>GPTEEQAAENWRDAMKTELQTIRTEIQEETARRQEELNAQNLVKMQELMSNFFQKITI[8x]

C. elegans SAS-6 physically interacts with SAS-5, a protein that shuttles rapidly between the cytoplasm and centrioles throughout the cell cycle. The presence of SAS-6 and SAS-5 at centrioles is essential for formation of the central tube, a cylindrical structure at the core of the emerging centriole. Overall, these findings led us to conclude that the segment between residues 125–265 contains two independently folded domains and encompasses all structured elements of SAS-5.

Native crystals of SAS-5CC diffracted to 1.8 Å resolution, whilst phases for structure solution were determined by single anomalous dispersion (SAD) using trimethyl lead acetate derivatized crystals. The structure of SAS-5CC suggested a parallel trimeric coiled coil, although this arrangement is distorted by crystal packing that intercalates the ends of successive triple helical bundles. To correct for these distortions, we performed molecular dynamics (MD) simulations starting from the crystallographic structure of SAS-5CC, which rapidly converged to a trimeric coiled-coil structure. SEC-MALS analysis of a slightly longer coiled-coil construct (SAS-5CC-L, residues 101–206) demonstrated formation of a trimer in solution in a concentration-dependent manner, with apparent Kd of ∼3 μM. Both the crystallographic model and MD simulations show a series of hydrophobic residues (W133, M137, L141, I144, I148, L159, M167 and M171) forming the core of the coiled coil and enabling trimer formation. Interestingly, we found that all these residues are conserved or conservatively substituted in SAS-5 homologs in other Caenorhabditis species, suggesting functional relevance. Taken together, these data support the notion that the SAS-5 coiled coil promotes the association of protein dimers towards higher-order assemblies. We found that the thermal unfolding profile of a SAS-52–265 L141E mutant showed a reduction in stability of the coiled coil by approximately 25°C, whereas stability of the Implico domain was not affected. Substituting an additional core hydrophobic residue of the coiled coil (SAS-52–265 L141E/M167E) effectively abrogated coiled coil formation, again with no effect on the Implico domain. As anticipated, coiled coil disruptions in either SAS-52–265 L141E or L141E/M167E mutants yielded a stable dimer in SEC-MALS experiments, mediated by the Implico domain.>[2x]VPKIVDHDERRRALADAVLALIAREGISAVTT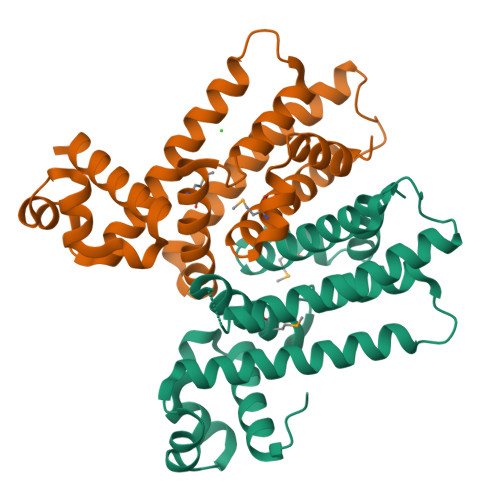RAVAEESGWSTGVLNHYFGSRHELLLAALRRAGDIQGDRYRTILDEEGAGPIEKLRNITASILPLDERRLAMTRVFLFFYAEGAAEETARGEIAAFLARWRGVVRESVVAAQREGTVSTDLDADAVTVALVALTDGLALQAILDPVVMKAISAEDAAARCVDAAVRRTTEEAGAVGR> MGSDKIHHHHHHMAHIFVYGTLKRGQPNHKVMLDHSHGLAAFRGRGCTVESFPLVIAGEHNIPWLLYLPGKG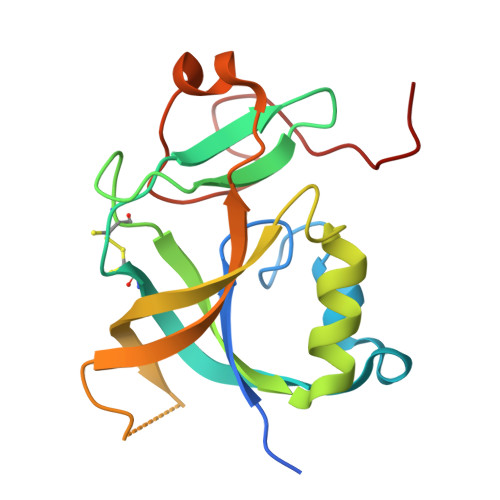HCVTGEIYEVDEQMLRFLDDFEDCPSMYQRTALQVQVLEWEGDGDPGDSVQCFVYTTATYAPEWLFLPYHESYDSEGPHGLRYNPRENR NICOTINATE MONONUCLEOTIDE | C11 H14 N O9 P | 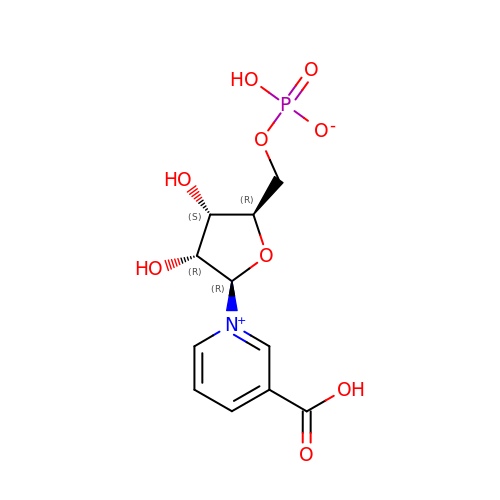JOUIQRNQJGXQDC-ZYUZMQFOSA-N>[8x]DYKDDDDKLVPRGSCHPRLSLHRPALEDLLLGSEANLTCTLTGLRDASGATFTWTPSSGKSAVQGPPERDLCGCYSVSSVLPGCAQPWNHGETFTCTAAHPELKTPLTANITKSGNTFRPEVHLLPPPSEELALNELVTLTCLARGFSPKDVLVRWLQGSQELPREKYLTWASRQEPSQGTTTYAVTSILRVAAEDWKKGETFSCMVGHEALPLAFTQKTIDRLAGKPTHINVSVVMAEADGTCY;> KSPIFGPEEVNSVEGNSVSITCYYPPTSVNRHTRKYWCRQGARGGCITLISSEGYVSSKYAGRANLTNFPENGTFVVNIAQLSQDDSGRYKCGLGINSRGLSFDVSLEVSQGPGLLNDTKVYTVDLGRTVTINCPFKTENAQKRKSLYKQIGLYPVLVIDSSGYVNPNYTGRIRLDIQGTGQLLFSVVINQLRLSDAGQYLCQAGDDSNSNKKNADLQVLKPEPELVYEDLRG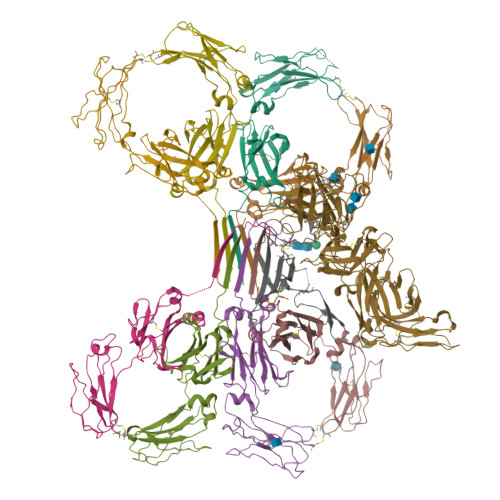SVTFHCALGPEVANVAKFLCRQSSGENCDVVVNTLGKRAPAFEGRILLNPQDKDGSFSVVITGLRKEDAGRYLCGAHSDGQLQEGSPIQAWQLFVNEESTIPRSPTVVKGVAGGSVAVLCPYNRKESKSIKYWCLWEGAQNGRCPLLVDSEGWVKAQYEGRLSLLEEPGNGTFTVILNQLTSRDAGFYWCLTNGDTLWRTTVEIKIIEGEPNLKVPGNVTAVLGETLKVPCHFPCKFSSYEKYWCKWNNTGCQALPSQDEGPSKAFVNCDENSRLVSLTLNLVTRADEGWYWCGVKQGHFYGETAAVYVAVEERKAAGSRDVSLAKADAAPDEKVLDSGFREIENKAIQDPRHHHHHH;> QEDERIVLVDNKCKCARITSRIIRSSEDPNEDIVERNIRIIVPLNNRENISDPTSPLRTRFVYHLSDLCKKCDPTEVELDNQIVTATQSNICDEDSATETCYTYDRNKCYTAVVPLVYGGETKMVETALTPDACYPD tert-butyl [(2S)-2-(2,5-difluorophenyl)-3-(quinolin-3-yl)propyl]carbamate | C23 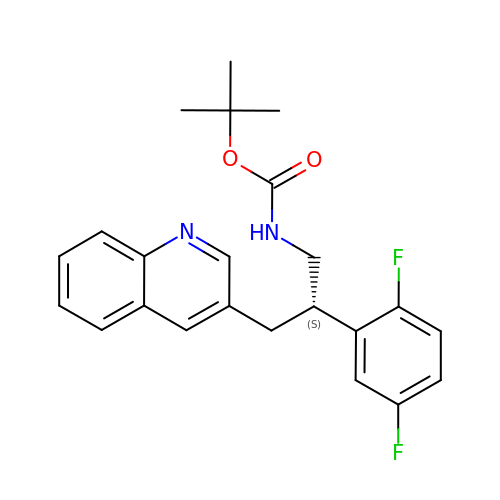H24 F2 N2 O2 | IRFHMTUHTBSEBK-QGZVFWFLSA-N> GMKNVTKASIDDLDSIVHIDIDVIGNDSRRNYIKHSIDEGRCVIVKEDNSISGFLTYDTNFFDCTFLSLIIVSPTKRRRGYASSLLSYMLSHSPTQKIFSSTNESNESMQKVFNANGFIRSGIVENLDEGDPEIIFYTKK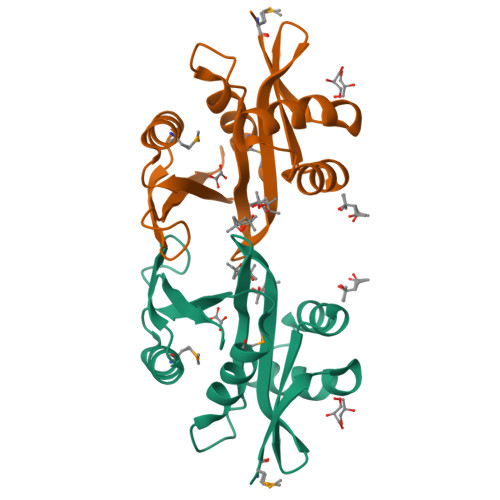LRA> MNDIVKSAWASVKMNTDFICVDTYSGYRSNQLDPLGV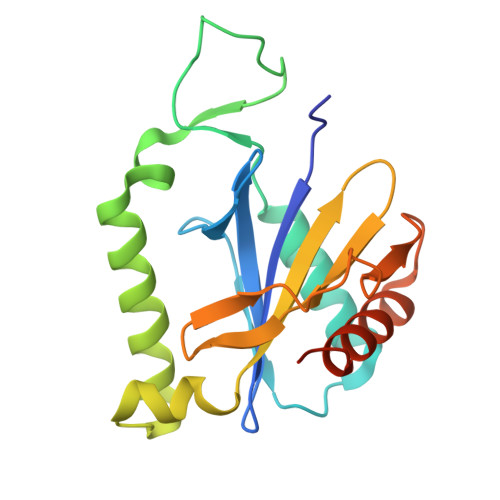QHLSSPDVSDLDLGEMVKDALSHSRFVLPAPRTDIWIHPEVTFDLDLYDSRRTVERYDEWVKKLMVHYGYKTKRALFKDMKSCDICCNHDAITISPTRHEKLEVWGGTGLKGSDNVILSVDSSPTEIGAGLRLALSRCKGLEHHHHHH>[2x]MIFTLRPYQQEAVDATLNHFRRHKTPAVIVLPTGAGKSLVIAELARLARGRVLVLAHVKELVAQNHAKYQALGLEADIFAAGLKRKESHGKVVFGSVQSVARNLDAFQGEFSLLIVDECHRIGDDEESQYQQILTHLTKVNPHLRLLGLTATPFRLGKGWIYQFHYHGMVRGDEKALFRDCIYELPLRYMIKHGYLTPPERLDMPVVQYDFSRLQAQSNGLFSEADLNRELKKQQRITPHIISQIMEFAATRKGVMIFAATVEHAKEIVGLLPAEDAALITGDTPGAERDVLIENFKAQRFRYLVNVAVLTTGFDAPHVDLIAILRPTESVSLYQQIVGRGLRLAPGKTDCLILDYAGNPHDLYAPEVGTPKGKSDNVPVQVFCPACGFANTFWGKTTADGTLIEHFGRRCQGWFEDDDGHREQCDFRFRFKNCPQCNAENDIAARRCRECDTVLVDPDDMLKAALRLKDALVLRCSGMSLQHGHDEKGEWLKITYYDEDGADVSERFRLQTPAQRTAFEQLFIRPHTRTPGIPLRWITAADILAQQALLRHPDFVVARMKGQYWQVREKVFDYEGRFRLAHELRG

In prokaryotes, the RadD protein is important for survival under conditions that include DNA-damaging radiation. The presence of conserved “helicase” motif sequences and the overall structure of RadD place it in the RecQ-like subgroup of the SF2s, which typically contain two RecA-like helicase domains followed by a zinc-binding region and a unique C-terminal domain. RadD binds branched DNA substrates and interacts with single-stranded DNA (ssDNA) binding protein (SSB), consistent with possible RadD involvement in processing branched DNA substrates such as replication forks or DNA repair intermediates. Recent work has revealed that RadD is an accessory protein for RecA, accelerating RecA-mediated DNA strand exchange only in the presence of RecA.

E. coli RadD was purified, crystallized in the presence of 1 mM ATPγS, and its structure was determined to 2.03-Å resolution using the structure of apo RadD as a molecular replacement search model. Thus, ADP was modelled in the RadD active site and we presume that it was produced by slow hydrolysis of ATPγS. With two major exceptions, the ADP-bound RadD was quite similar to the previously published structure of apo RadD. Most notably, the new structure resolved a second zinc-binding motif that was not modelled in the prior apo RadD structure. The present higher-resolution ADP-bound RadD structure shows unambiguously that RadD contains two zinc fingers, designated as ZF1 and ZF2. ZF1 contains cysteine residues 384, 387, 411 and 425, which comprise a variant zinc ribbon domain composed of two zinc-knuckles formed from the β1-β2 loop and the stem of an antiparallel beta hairpin formed by β4 and β5. ZF2 has a typical zinc-ribbon formation composed of two zinc-knuckles coordinating zinc through cysteine residues 434, 437, 448, and 451. In addition to the classical helicase motifs, the ADP-bound RadD structure identified a motif N-terminal to motif I that interacts with the adenine base of ADP. The RadD Q motif binds ADP through Gln9 and Arg6, where Gln9 hydrogen bonds with N6 and N7 of adenine and Arg6 stabilizes the interaction of ADP by Π-stacking the nitrogenous base. RadD motif I, also known as the Walker A motif or P-loop, primarily binds the α- and β-phosphates through backbone interactions whereas motif I Lys37 is poised to stabilize the presumed γ-phosphate position of ATP.> MGSMSLPEILPLEVIDKTINQKVLIVLQSNREFEGTLVGFDDFVNVILEDAVEWLIDPEDESRNEKVMQHHGR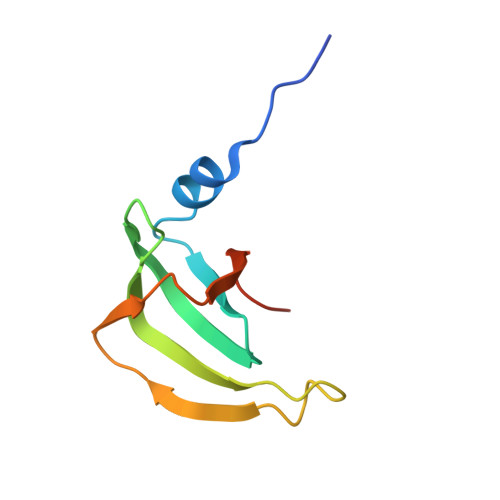MLLSGNNIAILVPGGKKTPTEAL> GESRDCHGTICHPVNEFCYVATERCHPCIEVCN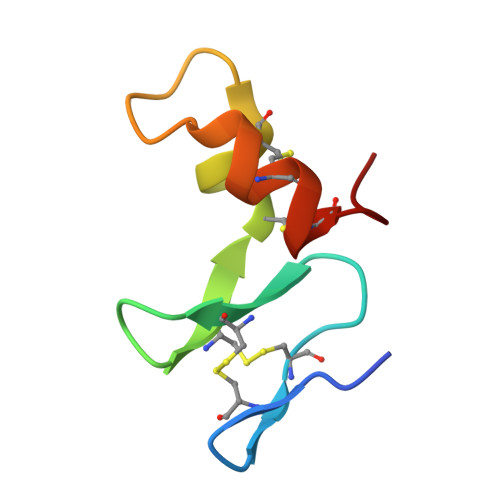NQTHNYDAFLCAKECSAYK> MLFTRCLLAVTTINSSTASAAGRLIRIRKKSKWIDRRSKRIPHNGKDVWQFGEQ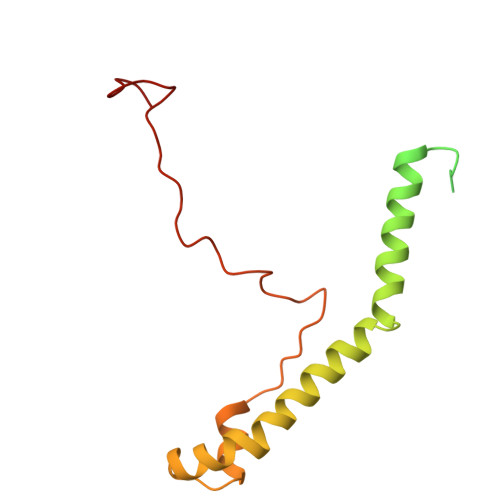PSCALCHVRFRFKQDYEAHKESELHQNRLRWVETMKWWEEIGEPHHQQHAASEWEWFRQRVLPAKAAAMGLSEEDAARELRRAVMHETPRWYSRIQPPNARSEIKEPRDQRWPSSPKW> LEHHHHHMVDNRMRFTIDQNMQFPLVEIDLEHGGSVYLQQGSMVYHTENVTLNTKLNGKGSGLGKLVGAIGRSMVSGESMFITQAMSNGDGKLALAPNTPGQIVALELGEKQYRLNDGAFLALDGSAQYKMERQNIGKALFGGQGGLFVMTTEGLGTLLANSFGSIKKITLDGGTMTIDNAHVVAWSRELDYDIHLEN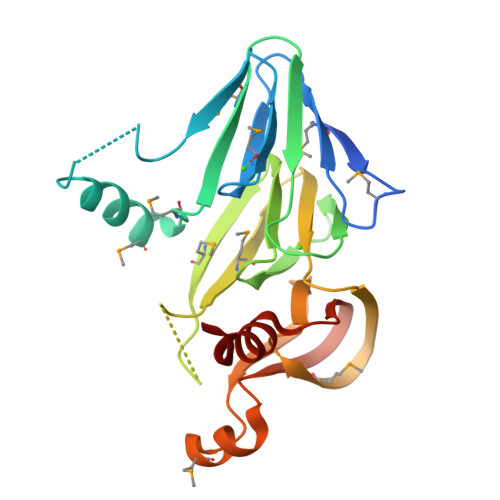GFMQSIGTGEGVVNTFRGHGEIYIQSLNLEQFAGTLKRYLPTSSN> GSGEVTCEPGTTFKDKCNTCRCG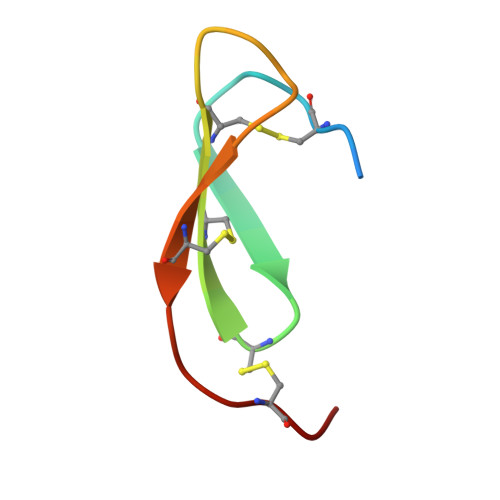SDGKSAFCTRKLCYQ>MKGPYKHFMQKEIFEQPDSAFNTMRGRIDFENCVVTLGGLKSWLSTIRRCRRIIMIACGTSYHSCLATRSIFEELTEIPVSVELASDFLDRRSPVFRDDTCVFVSQSGETADSILALQYCLERGALTVGIVNSVGSSMSRQTHCGVHINAGPEIGVASTKAYTSQYIALVMFALSLSNDSISRKGRHEEIIKGLQKIPEQIKQVLKLENKIKDLCNSSLNDQKSLLLLGRGYQFATALEGALKIKEISYMHSEGVLAGELK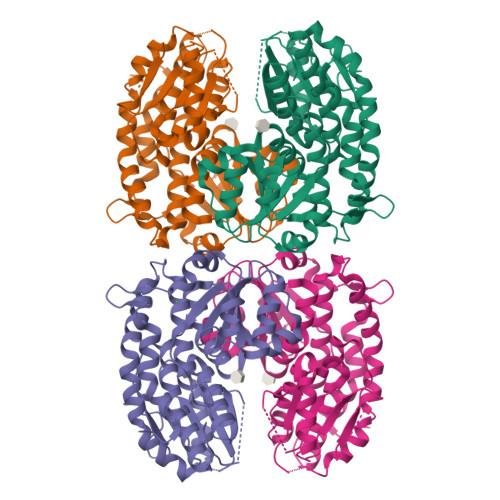HGILALVDEDLPIIAFATRDSLFPKVMSAIEQVTARDGRPIVICNEGDAIISNDKVHTTLEVPETVDCLQGLLNVIPLQLISYWLAVNRGIDVDFPRNLAKSVTVE[2x]> LSTTARRTKVTLPDLKWDFGALEPYISGQINELHYTKHHQTYVNGFNTAVDQFQELSDLLAKEPSPANARKMIAIQQNIKFHGGGFTNHCLFWENLAPESQGGGEPPTGALAKAIDEQFGSLDELIKLTNTKLAGVQG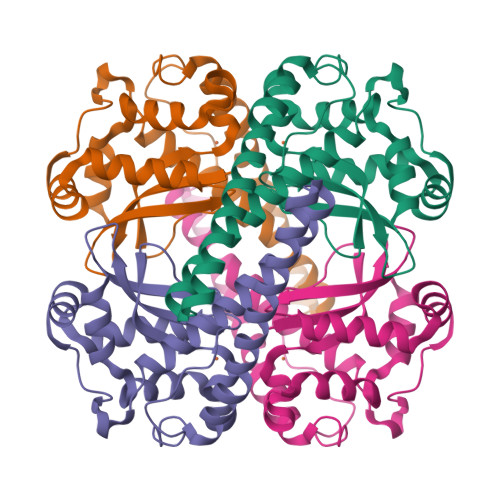SGWAFIVKNLSNGGKLDVVQTYNQDTVTGPLVPLVAIDAWEHAYYLQYQNKKADYFKAIWNVVNWKEASRRFDAGKI>[2x]MGGSHHHHHHLESTSLYKKSSSTPPRGVTVVNNFDCKRYLGTWYEIARFDHRAERGLEKVTATYSLRDDGGLNVIFKGYNPDRGMWQQYVGKAYFTGAPTRAALKVAFFGPFYGGYNVIALDREYRHALVCGPDRDYLWINSRTPTISDEVKQEMLAVATREGFDVSKFIWVQQPGS

Later, proteins capable of binding and increasing the fluorescent signals of fluorogenic molecules became commonly referred to as fluorogen activating proteins (FAPs). In silico shortlisting with the further screening of the lipocalin Blc mutants launched DiBs FAPs tags family binding green and red BODIPY dyes. It suggests that the easier task of fine-tuning the fluorogen-binding properties of an already functional protein in silico should be readily achievable. To test this hypothesis, we used Rosetta for computational ligand docking followed by protein binding pocket redesign to further improve the previously described FAP DiB1 that is capable of binding to a BODIPY-like dye M739. The designed protein, DiB-RM, shows higher brightness, localization precision, and apparent photostability in protein-PAINT super-resolution imaging compared to its parental variant DiB1.

The resulting protein, designated DiB-RM, performs better than its parental variant both in vitro (except for the dissociation constant) and as a tag for protein-PAINT with higher brightness, localization precision, and apparent photostability. We speculate that the observed decrease in affinity to the ligand is caused by introducing two aromatic amino acids in the protein’s binding pocket (76F and 89Y). While the presence of these amino acids is most likely responsible for the observed increased brightness of the DiB-RM:M739 complex compared to the parental DiB1:M739 through the better protein:ligand interface packing, in the absence of the ligand these bulky amino acids might partially hinder the entrance of the ligand in the binding pocket. Crystallization analysis of DiB-RM in the apo form in different conditions further confirmed the already known high flexibility of the E/F lipocalin loop that was not properly addressed during our computational redesign. (C) The side and the top views on the overlay of the DiB1 complex (shown in yellow) with the DiB-RM apo structure (shown in light gray). The side chains of the amino acids in the positions that differ between DiB1 and DiB-RM as well as M739 are shown as sticks. Interestingly, in both cases, the 50 top-scored structures contained a mixture of different ligand positions one of which was matching the chromophore position in DiB1 while the other was very close to our original docked pose. This observation together with our inability to obtain the DiB-RM:M739 co-crystal structure might indicate that we have stabilized an alternative binding site for the ligand by the introduced mutations but have not destroyed the other one. As a result, the ligand in DiB-RM might have multiple possible binding positions. This can also explain the larger apparent dissociation constant of this new complex. Rigidifying of this loop through shortening or designed interactions can provide better stabilization of the ligand in the binding pocket.>[2x]M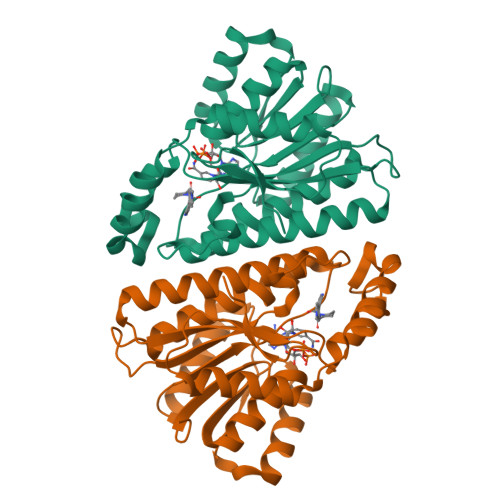VNGKVALVTGAAQGIGRAFAEALLLKGAKVALVDWNLEAGVQCKAALDEQFEPQKTLFIQCDVADQQQLRDTFRKVVDHFGRLDILVNNAGVNNEKNWEKTLQINLVSVISGTYLGLDYMSKQNGGEGGIIINMSSLAGLMPVAQQPVYCASKHGIVGFTRSAALAANLMNSGVRLNAICPGFVNTAILESIEKEENMGQYIEYKDHIKDMIKYYGILDPPLIANGLITLIEDDALNGAIMKITTSKGIHFQDY In Rhodobacter sphaeroides, TakP (previously named SmoM) is an ESR from a TRAP transporter and binds α-keto acids in vitro. In this paper, we present the high resolution structures of TakP in its unliganded form and complexed with sodium-pyruvate. This study reveals a key role for an ion in the attachment mode of the substrate, as well as an unexpected dimerization largely mediated by a helix swapping. Thus, and despite very low sequence similarity, the TakP fold is characteristic of a type II ESR.

The structure of the selenomethionine-labeled protein in its native form was first solved by the MAD method and then refined to 2.0 Å resolution with an R-factor of 17.9% (Rfree = 20.5%). After a successful co-crystallization of TakP with pyruvate, the structure of the protein-substrate complex was solved by molecular replacement and refined to 1.4 Å resolution (R = 17.3%, Rfree = 18.4% ; Table 1 and Additional file 1 for an assessment of the quality of the electron density map). In the second crystal form obtained with the substrate-bound protein, the asymmetric unit contains one dimer with both monomers now found in the closed configuration. In the cleft between domains I and II of each monomer an extra electron density was unambiguously assigned to an ion-pyruvate complex. In the complex structure, the acidic moiety of the pyruvate is involved in a salt bridge with Arg177 and one oxygen atom is H-bonded to Tyr100. The central feature for the binding of the pyruvate to the protein is the presence of a cation. This cation has a bi-pyramidal coordination with a square base. The four equatorial positions are provided by the O3 of pyruvate, the main chain carbonyl oxygen of Trp215 and a bi-dentate and mono-dentate ligand provided by the side chains of Glu214 and Glu240, respectively. The apical positions are occupied on one side by an oxygen atom from the acidic moiety of pyruvate and, on the other side, by the Oδ1 of the side chain of Gln156. Since only sodium salts were present in our crystallization conditions this cation can be safely identified as a sodium ion. Among the six residues involved in the recognition of sodium-pyruvate, only one (Tyr100) is provided by domain I, while the others belong to domain II or to the hinge.

>[2x]MDRRSFITKAAVGGAAASALAAPALAQSAPKVTWRLASSFPKSLDTIFGGAEVLSKMLSEATDGNFQIQVFSAGELVPGLQAADAVTEGTVECCHTVGYYYWGKDPTFALAAAVPFSLSARGINAWHYHGGGIDLYNEFLSQHNIVAFPGGNTGVQMGGWFRREINTVADMQGLKMRVGGFAGKVMERLGVVPQQIAGGDIYPALEKGTIDATEWVGPYDDEKLGFFKVAPYYYYPGWWEGGPTVHFMFNKSAYEGLTPTYQSLLRTACHAADANMLQLYDWKNPTAIKSLVAQGTQLRPFSPEILQACFEAANEVYAEMEASNPAFKKIWDSIKAFRSEHYTWAQIAEYNYDTFMMVQQNAGKL>HMKTSDPLKILANADTMKVLGVQRPLLQSTIIVEKTVQDLMNLMHDLSAYSDQFLNMVCVKLQEYKDTCSTAYRGIVQSEEKLVISASWAKDDDISRLLKSLPNWTNMAQPKQLRPKREEEEDFIRAAFGKESEVLIGNLGDKLIPPQDILRDVSDLKALANMHESLEWLAGRTKSAFSSLSASQMLSPAQESHVNMDLPPVSEQIMQTLSELAKSFQDMADRCLLVLHLEVRVHCFHYLIPLAKEGNYAIVANVESMDYDPLVVKLNKDISAMEEAMSASLQQHKFQYIFEGLGHLISCILINGAQYFRRISESGIKKMCRNIFVLQQNLTNITMSREADLDFARQYYE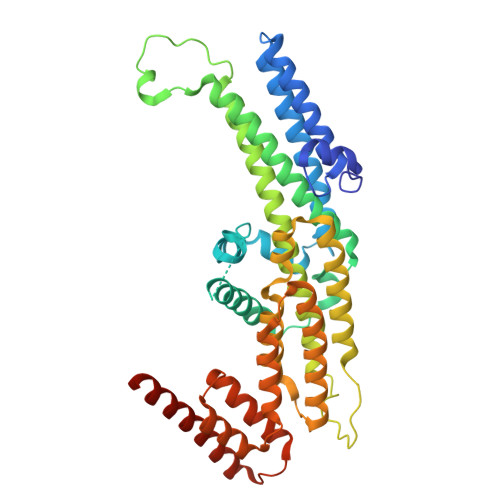MLYNTADELLNLVVDQGVKYTELEYIHALTLLHRSQTGVGDQTTQNTRLQRLKEIICEQAAIKQATKDKKITTV[2x]The lipid-enveloped bacteriophages of the Cystoviridae family infect Gram-negative bacteria, mainly plant-pathogenic Pseudomonas species and share similarities with the members of the Reoviridae family, including bluetongue virus and rotavirus. Their genome of ∼14 kb consists of three dsRNA segments small (S), medium (M) and large (L), which are sequentially encapsidated as ssRNA precursors into the icosahedrally symmetric procapsid by the packaging NTPase P4 (15–23). P4 is a protein of ∼35 kDa, which can assemble into a hexameric ring. NTP-binding sites are located on the external perimeter of the ring at the interfaces between adjacent subunits, whereas the nucleic acid binding sites are found in the central channel. P4 proteins are the only known RNA-specific helicases belonging to helicase Superfamily 4 (SF4).

All P4 proteins form a hexameric ring with a central channel varying in size from 13 to 21 Å (30 Å for ɸ8 P4Δ281) and external diameter of ∼100 Å. The deletion of the C-terminal portion of the protein (residues 282–321) more than doubles the diameter of the central channel (from 13 to 30 Å), as the C-terminus wraps upwards from the base of the hexamer, along the inter-subunit cleft, to stick down into the central channel. As the C-terminal domain is (i) necessary for ATP hydrolysis (data not shown), (ii) restricts the diameter of the central channel and (iii) blocks the interface through which RNA is thought to be loaded, we postulate that the C-terminal region needs to be displaced by RNA for ring opening and subsequent ATP hydrolysis to occur. The ɸ8 P4 ATPase activity is tightly coupled to ssRNA translocation, as it will only hydrolyse ATP in the presence of ssRNA. The ɸ8 P4 N-terminal domain is composed of two helices separated by a four-stranded antiparallel β-sheet. However, in ɸ8 P4, these residues are displaced >8 Å from that position and therefore cannot contribute to catalysis. This suggests that in ɸ8 P4, extensive conformational changes occur as a consequence of nucleotide and/or oligonucleotide binding, which render the enzyme competent for catalysis. Nevertheless, the L1 loop contains a motif (LKK) that has been shown to be crucial for RNA binding. The first lysine of this motif (K185) is found in the equivalent position to K241 of ɸ12 P4 and is also seen interacting with D220 of loop L2.

>[6x]MARKTKVTPDDNSIIDLGPRVQSLMEQLATTKLEEGVKNLDMGSVYEITTVMVLGNSILGFHKGDLVKMVRPSVSARDLIGVGYATASAAVVRQRLIEHKIEAGAELIISGTAGGKTVLTNHYAAQMCAKGLKVAVVSMAEAERPLYGSVLHVFAALHLAAVSDVDVLYVDSLRSVYNELGGNLKKGGVSRQVDGMLTALDQYARAVNMRVVFTLNPSDDENVDAAVRSVFKTASASMHTARRIKSFAVNGTAFTAETEIHLRADRSNSANRVSGDLVSR> GSMEDVEIKPRGYQLRLVDHLTKSNGIVYLPTGSGKTFVAILVLKRFSQDFDKPIESGGKRALFMCNTVELARQQAMAVRRCTNFKVGFYVGEQGVDDWTRGMWSDEIKKNQVLVGTAQVFLDMVTQTYVALSSLSVVIIDECHHGTGHHPFREFMRLFTIANQTKLPRVVGLTGVLIKGNEITNVATKLKELEITYRGNIITVSDTKELENVMLYATKPTEVMVSFPHQEQVLTVTRLISAEIEKFYVSLDLMNIGVQPIRRSKSLQCLRDPSKKSFVKQLFNDFLYQMKEYGIYAASIAIISLIVEFDIKRRQAETLSVKLMHRTALTLCEKIRHLLVQKLQDMTYDDDDDNVNTEEVIMNFSTPKVQRFLMSLKVSFADKDPKDICCLVFVERRYTCKCIYGLLLNYIQSTPELRNVLTPQFMVGRNNISPDFESVLERKWQKSAIQQFRDGNANLMICSSVLEEGIDVQACNHVFILDPVKTFNMYVQSKGRARTTEAKFVLFTADKEREKTIQQIYQYRKAHNDIAEYLKDRVLEKTEPELYEIKGHFQDDIDPFTNENGAVLLPNNALAILHRYCQTIPTDAFGFVIPWFHVLQEDERDRIFGVSAKGKHVISINMPVNCMLRDTIYSDPMDNVKTAKISAAFKACKVLYSLGELNERFVPKTLKERVASIADVHFEHWNKYGDSVTATVNKADKSKDRTYKTECPLEFYDALPRVGEICYAYEIFLEPQFESCEYTEHMYLNLQTPRNYAILLRNKLPRLAEMPLFSNQGKLHVRVANAPLEVIIQNSEQLELLHQFHGMVFRDILKIWHPFFVLDRRSKENSYLVVPLILGAGEQKCFDWELMTNFRRLPQSHGSNVQQREQQPAPRPEDFEGKIVTQWYANYDKPMLVTKVHRELTPLSYMEKNQQDKTYYEFTMSKYGNRIGDVVHKDKFMIEVRDLTEQLTFYVHNRGKFNAKSKAKMKVILIPELCFNFNFPGDLWLKLIFLPSILNRMYFLLHAEALRKRFNTYLNLHLLPFNGTDYMPRPLEIDYSLKRNVDPLGNVIPTEDIEEPKSLLEPMPTKSIEASVANLEITEFENPWQKYMEPVDLSRNLLSTYPVELDYYYHFSVGNVCEMNEMDFEDKEYWAKNQFHMPTGNIYGNRTPAKTNANVPALMPSKPTVRGKVKPLLILQKTVSKEHITPAEQGEFLAAITASSAADVFDMERLEILGDSFLKLSATLYLASKYSDWNEGTLTEVKSKLVSNRNLLFCLIDADIPKTLNTIQFTPRYTWLPPGISLPHNVLALWRENPEFAKIIGPHNLRDLALGDEESLVKGNCSDINYNRFVEGCRANGQSFYAGADFSSEVNFCVGLVTIPNKVIADTLEALLGVIVKNYGLQHAFKMLEYFKICRADIDKPLTQLLNLELGGKKMRANVNTTEIDGFLINHYYLEKNLGYTFKDRRYLLQALTHPSYPTNRITGSYQELEFIGDAILDFLISAYIFENNTKMNPGALTDLRSALVNNTTLACICVRHRLHFFILAENAKLSEIISKFVNFQESQGHRVTNYVRILLEEADVQPTPLDLDDELDMTELPHANKCISQEAEKGVPPKGEFNMSTNVDVPKALGDVLEALIAAVYLDCRDLQRTWEVIFNLFEPELQEFTRKVPINHIRQLVEHKHAKPVFSSPIVEGETVMVSCQFTCMEKTIKVYGFGSNKDQAKLSAAKHALQQLSKCDA;> GPFTMDNKSAVSALQEFCARTQINLPTYSFIPGEDGGYVCKVELLEIEALGNGRSKRDAKHLAASNILRKIQLLPGIHGLMKDSTVGDLDEELTNLNRDMVKELRDYCVRREMPLPCIEVVQQSGTPSAPEFVACCSVASIVRYGKSDKKKDARQRAAIEMLALISSNSDNLRPDQMQVASTSKLKVVDMEESMEELEALRRKKFTTYWELKEAGSVDHT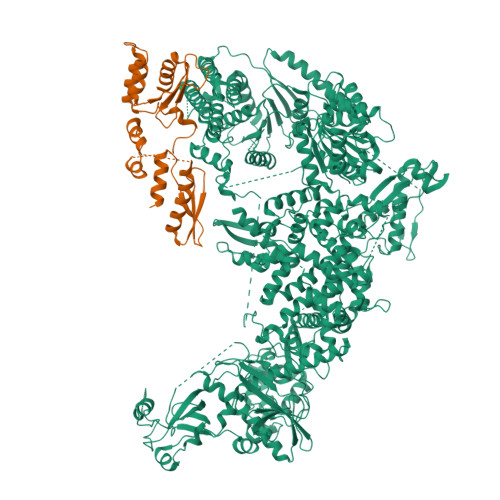GMRLCDRHNYFKNFYPTLKKEAIEAINSDEYESSKDKAMDVMSSLKITPKISEVESSSLVPLLSVELNCAFDVVLMAKETDIYDHIIDYFRTMLI> MAAESSTSTVSNLATMATVTASGREVSSGFGPELAADNQDLPDNPTDKSVHNASGASRWSADRGSGPWWLAYEFPGEATISSVNIAWGNTYATNYSIQTSDDGSNWTDVKTGLKATAQAQWVKTTFDTPIKTRHIRMIATTKSQSWSLSVWEMRTMGTISAVATDPLSRLTPRPLYAQSADGEAFELKKNTCVSVSDGSLLPAVDVMRDELGTSYGLKLAEGTNCPITFTLDENLDVTGHVGSAQSITADEAYTIVSDADSVTVKARSATAGIWAAQTLLQLIGPWTNSTVKLADVAFIPAVNIADAPRYQWRGVLVDPARSFYPLDEMKQMIDVMSAYKMNTLHLHLSEDEGFRVEITNDGRADGDTTDYTQLAIKSGAISYQSAWTSNWSPAQDGRTGYWTQSEFIELVAYAADHGIAIVPEIDGPGHSFSLLHGLAELNTGNSNPKPAAGEDTPAFIQSAQGRSSLATDADITYTVLGHIMDQLDGMIDKGIKASTMPASELKRMYFHLGGDELFLSGGAGNKTERLQEYLGRSGALVKERDKTTIVWNDGLDAVDQIPEGSVVQHWTGNAANNASIQKLLNQRNGKIIMSPAGNTYFPQRPGTETTGVTWACGACTTSNFYQWNPTSSAGTTEDKVLGVEDALWSEHLRSLNDAEFLMYTRMMATAEVGWT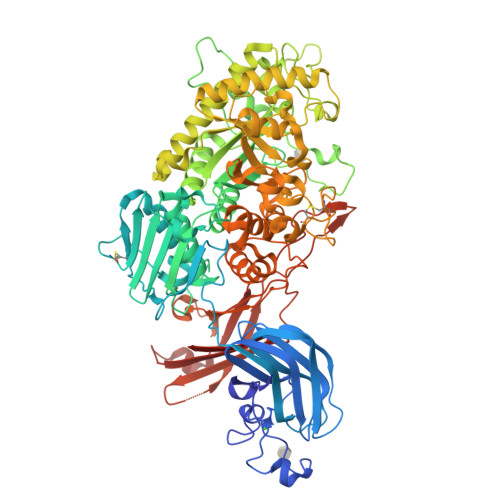QQNRKDYDNWNKRVGDIAIDLMNRGANFHKATEVTSWKGSYAAVDAAEQKVTDGKVLVGRYAEPGLTGTDGLSFTATYTAEGGTAVNLPVTPDMKQTYSQQQLKNGRLVVNGAHMNSIVDVYVTLPSDVLAADSEAVGRLDVSVSSSTYHHHHHH4-amino-N-(piperidin-4-yl)-1,2,5-oxadiazole-3-carboxamide | C8 H13 N5 O2 | 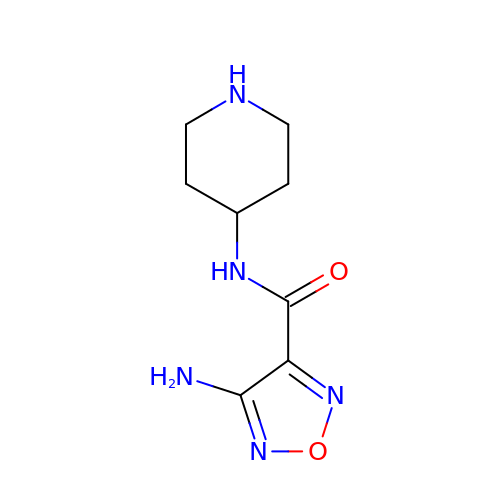LGMVLTCRFMCVHB-UHFFFAOYSA-N> MKVAGGLELGAAALLSASPRALVTLSTGPTCSILPKNPLFPQNLSSQPCIKMEGDKSLTFSSYGLQWCLYELDKEEFQTFKELLKKKSSESTTCSIPQFEIENANVECLALLLHEYYGASLAWATSISIFENMNLRTLSEKARDDMKRHSPEDPEATMTDQGPSKEKVPGISQAVQQDSATAAETKEQEISQAMEQEGATAAETEEQEISQAMEQEGATAAETEEQGHGGDTWDYKSHVMTKFAEEEDVRRSFENTAADWPEMQTLAGAFDSDRWGFRPRTVVLHGKSGIGKSALARRIVLCWAQGGLYQGMFSYVFFLPVREMQRKKESSVTEFISREWPDSQAPVTEIMSRPERLLFIIDGFDDLGSVLNNDTKLCKDWAEKQPPFTLIRSLLRKVLLPESFLIVTVRDVGTEKLKSEVVSPRYLLV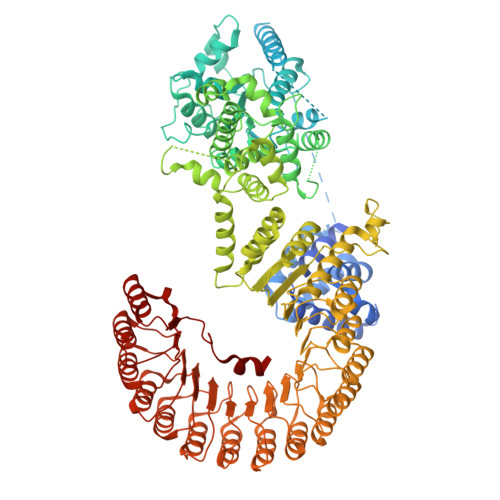RGISGEQRIHLLLERGIGEHQKTQGLRAIMNNRELLDQCQVPAVGSLICVALQLQDVVGESVAPFNQTLTGLHAAFVFHQLTPRGVVRRCLNLEERVVLKRFCRMAVEGVWNRKSVFDGDDLMVQGLGESELRALFHMNILLPDSHCEEYYTFFHLSLQDFCAALYYVLEGLEIEPALCPLYVEKTKRSMELKQAGFHIHSLWMKRFLFGLVSEDVRRPLEVLLGCPVPLGVKQKLLHWVSLLGQQPNATTPGDTLDAFHCLFETQDKEFVRLALNSFQEVWLPINQNLDLIASSFCLQHCPYLRKIRVDVKGIFPRDESAEACPVVPLWMRDKTLIEEQWEDFCSMLGTHPHLRQLDLGSSILTERAMKTLCAKLRHPTCKIQTLMFRNAQITPGVQHLWRIVMANRNLRSLNLGGTHLKEEDVRMACEALKHPKCLLESLRLDCCGLTHACYLKISQILTTSPSLKSLSLAGNKVTDQGVMPLSDALRVSQCALQKLILEDCGITATGCQSLASALVSNRSLTHLCLSNNSLGNEGVNLLCRSMRLPHCSLQRLMLNQCHLDTAGCGFLALALMGNSWLTHLSLSMNPVEDNGVKLLCEVMREPSCHLQDLELVKCHLTAACCESLSCVISRSRHLKSLDLTDNALGDGGVAALCEGLKQKNSVLARLGLKACGLTSDCCEALSLALSCNRHLTSLNLVQNNFSPKGMMKLCSAFACPTSNLQIIGLWKWQYPVQIRKLLEEVQLLKPRVVIDGSWHSFDEDDRYWWKN4-(pyridin-2-yl)benzoic acid | C12 H9 N 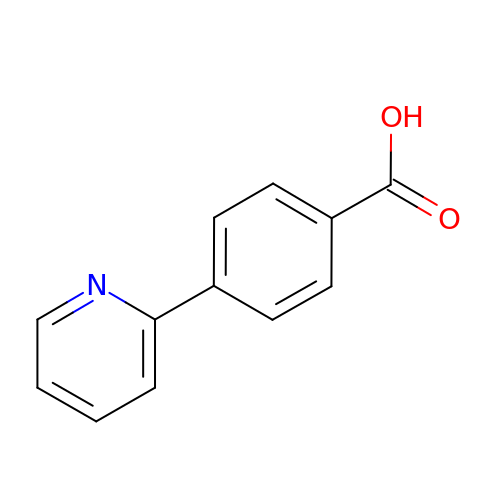O2 | AQIPNZHMXANQRC-UHFFFAOYSA-N> MHHHHHHGAQPARSANDTVVVGSIIFTEGIIVANMVAEMIEAHTDLKVVRKLNLGGYNVNFEAIKRGGANNGIDIYVEYTGHGLVDILGFPATTDPEGAYETVKKEYKRKWNIVWLKPLGFNNTYTLTVKDELAKQYNLKTFSDLAKISDKLILGATMWFLEGPDGYPGLQKLYNFKFKHTKSMDMGIRYTAIDNNEVQVIDAWATDGL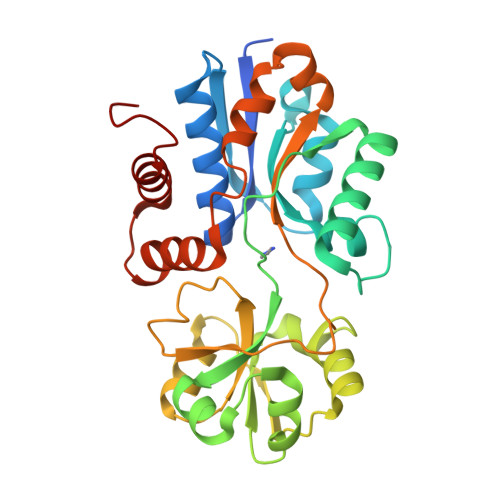LVSHKLKILEDDKAFFPPYYAAPIIRQDVLDKHPELKDVLNKLANQISLEEMQKLNYKVDGEGQDPAKVAKEFLKEKGLILQVD>[14x]MAENTKNENITNILTQKLIDTRTVLIYGEINQELAEDVSKQLLLLESISNDPITIFINSQGGHVEAGDTIHDMIKFIKPTVKVVGTGWVASAGITIYLAAEKENRFSL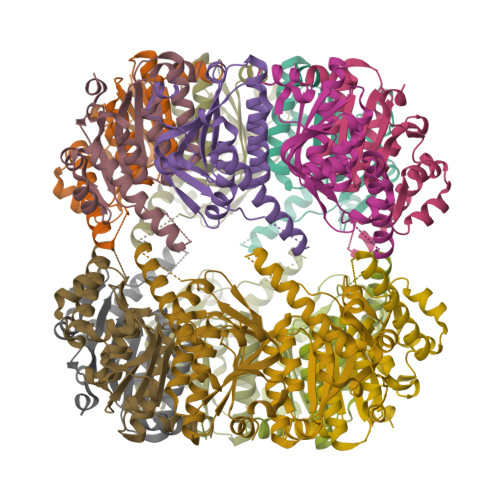PNTRYMIHQPAGGVQGQSTEIEIEAKEIIRMRERINRLIAEATGQSYEQISKDTDRDFWLSVNEAKDYGIVNEIIENRDGLKMASWSHPQFEK>MQSINFRTARGNLSEVLNNVEAGEEVEITRRGREPAVIVSKATFEAYKKAALDAEFASLF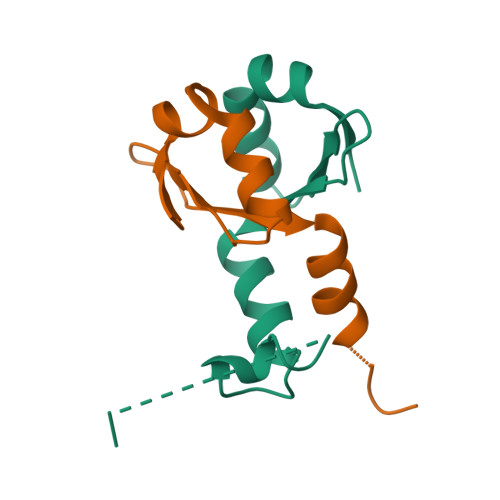DTLDSTNKELVNR[3x]> VNFEEVRELVPQKYPFLFIDKVIELQKEARIVCLKNISGNEPFFAGHFPDFAIMPGVLIVEALAQASIILFKKSFSTEQ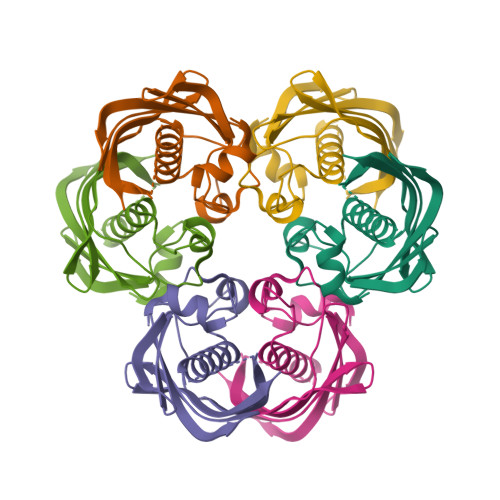HKDDVFLLASANVRFSKPVFPGDQLILEIDIEKVISSAAIVKGVAKVGDKVVTKATLSFGVA> MFSAGHKIKGTVVLMPKNELEVNPDGSAVDNLNAFLGRSVSLQLISATKADAHGKGKVGKDTFLEGINTSLPTLGAGESAFNIHFEWDGSMGIPGAFYIKNYMQVEFFLKSLTLEAISNQGTIRFVCNSWVYNTKLYKSVRIFFANHTYVPSETPAPLVSYREEELKSLRGNGTGERKEYDRIYDYDVYNDLGNPDKSEKLARPVLGGSSTFPYPRRGRTGRGPTVTDPNTEKQGEVFYVPRDENLGHLKSKDALEIGTKSLSQIVQPAFES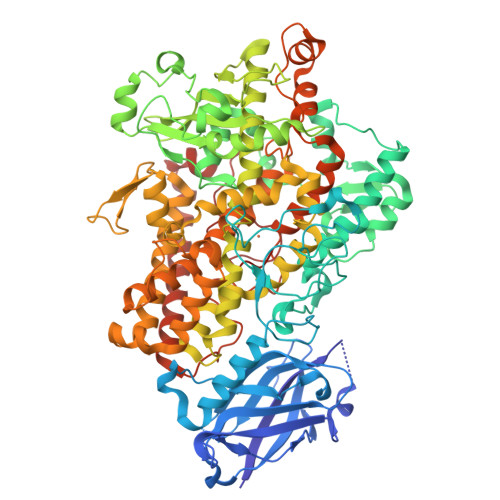AFDLKSTPIEFHSFQDVHDLYEGGIKLPRDVISTIIPLPVIKELYRTDGQHILKFPQPHVVQVSQSAWMTDEEFAREMIAGVNPCVIRGLEEFPPKSNLDPAIYGDQSSKITADSLDLDGYTMDEALGSRRLFMLDYHDIFMPYVRQINQLNSAKTYATRTILFLREDGTLKPVAIELSLPHSAGDLSAAVSQVVLPAKEGVESTIWLLAKAYVIVNDSCYHQLMSHWLNTHAAMEPFVIATHRHLSVLHPIYKLLTPHYRNNMNINALARQSLINANGIIETTFLPSKYSVEMSSAVYKNWVFTDQALPADLIKRGVAIKDPSTPHGVRLLIEDYPYAADGLEIWAAIKTWVQEYVPLYYARDDDVKNDSELQHWWKEAVEKGHGDLKDKPWWPKLQTLEDLVEVCLIIIWIASALHAAVNFGQYPYGGLIMNRPTASRRLLPEKGTPEYEEMINNHEKAYLRTITSKLPTLISLSVIEILSTHASDEVYLGQRDNPHWTSDSKALQAFQKFGNKLKEIEEKLVRRNNDPSLQGNRLGPVQLPYTLLYPSSEEGLTFRGIPNSISI Mitochondrial ATP synthase consists of the soluble F1 and membrane-bound Fo subcomplexes and occurs in dimers that assemble into oligomers to induce the formation of inner-membrane folds, called cristae. Dissociation of ATP synthase dimers into monomers results in the loss of native cristae architecture and impairs mitochondrial function. Here, we report cryo-EM structures of the intact ATP synthase dimer from Trypanosoma brucei in ten different rotational states. Although overall dimer architecture varies among eukaryotes, we find that subunit-g together with subunit-e form an ancestral oligomerization motif, which is shared between the trypanosomal and mammalian lineages.

Using masked refinements, maps were obtained for the membrane region, the rotor, and the peripheral stalk. The nucleotide base is inserted between two Arg82c residues, whereas the triphosphate region is coordinated by another five Arg82c residues, with Tyr79δ and Asn76δ providing asymmetric coordination contacts. The β-barrel, which has previously been reported also in the ATP synthase from E. gracilis, extends from the c10-ring approximately 15 Å to the lumen. The mechanism of proton translocation involves sequential protonation of E102 of subunits-c, rotation of the c10-ring with neutralized E102c exposed to the phospholipid bilayer, and release of protons on the other side of the membrane.

> MSGKLRLYKEKLEGYNRFYSIVKTIKMVTLAKYRAAQGRIRTRDFSLRYTELAFSKPQASRDAVVAAKNALVYIPITTNRGSCGALNSNIVRCIDSVVSSKMVLMPVGKRGIDSFSKLYPDEFRYGIINDMKESMHFGYATFVIENAYEVSKDADRYQVIFNRFVSAGVQRNAVYNIPSYEKWKEDLADAASSDNQKNRYLFANALQNEEEQLIRDFFDFHAALAVLNAVGENELSEQAARLVAVEGQLTNISSLQQRTSSLYNKTRQFGITAALIEILSAMSSLEGNAMKGVRRNKFWEGAVTK;> MFRTFGRRLVSCTLPLLQSAPHDLPEGFEFMEHKVVNKDIHAPHENLETLRLTLTRQDEFLLREEPVKCVTVTGTNGEYGIYPGHAYKIVQLNPSPLTVEYTDGTTKKYFVSGGFAHINNEGSCDVNTVECTLLDDLDLAIAEKELAAQQAALGSAKDDKAKSVVEIRISVIEAVIAALKHH;> MIRRSCALLSSSWRDHGISYLKYLNVCTETLHSTVKESRRAKYERWSKPCYTAQRPDGAGGQETIDKVPIHTKDY;>MMRRLALQSSIRRATPFATPLVASTKALNPMCSAITIREASTVAISVQGLHYVGTGLAAIALAGVGLGIGTIFGNLLVACARQPNLTKMLFNYAILGFALTEAIGLFALMLAFLMLFS[10x]>[2x]MDVTAKYELIGLMAYPIRHSLSPEMQNKALEKAGLPFT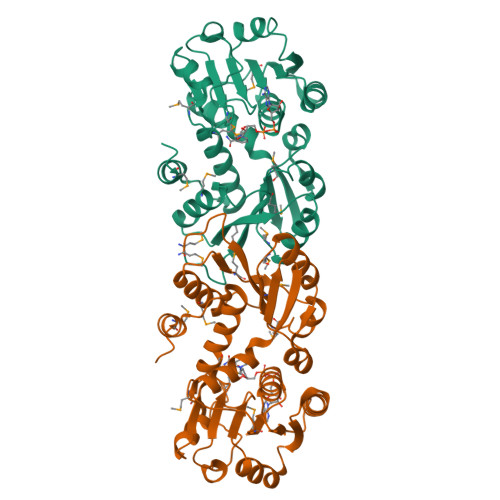YMAFEVDNDSFPGAIEGLKALKMRGTGVSMPNKQLACEYVDELTPAAKLVGAINTIVNDDGYLRGYNTDGTGHIRAIKESGFDIKGKTMVLLGAGGASTAIGAQGAIEGLKEIKLFNRRDEFFDKALAFAQRVNENTDCVVTVTDLADQQAFAEALASADILTNGTKVGMKPLENESLVNDISLLHPGLLVTECVYNPHMTKLLQQAQQAGCKTIDGYGMLLWQGAEQFTLWTGKDFPLEYVKQVMGFGA>SNAKSEIGKYAPFFSLPNAKGEKITRSSDAFKQKSLLINFWASWNDSISQKQSNSELREIYKKYKKNKYIGMLGISLDVDKQQWKDAIKRDTLDWEQVCDFGGLNSEVAKQYSI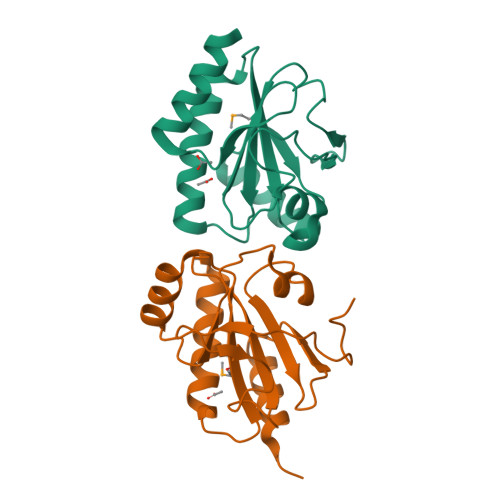YKIPANILLSSDGKILAKNLRGEELKKKIENIVEEA[4x]N-hydroxy-4-{[(propan-2-yl)(2,3,4,5-tetrafluorobenzene-1-sulfonyl)amino]methyl}benzamide | C17 H16 F4 N2 O4 S | 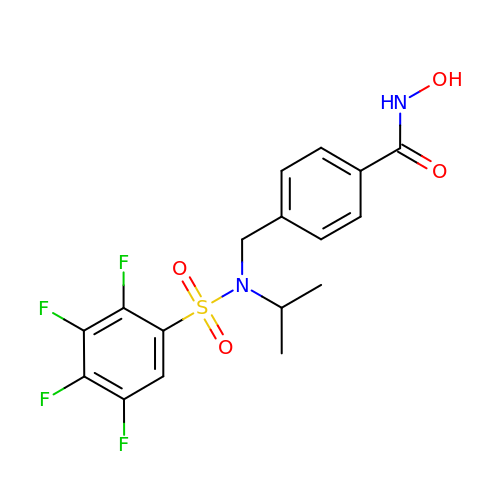SJWJGLIJTRUXIZ-UHFFFAOYSA-N>GMRPALYFCGSIRGGREDRTLYERIVSRLRRFGTVLTEHVAAAELGARGEEAAGGDRLIHEQNLEWLQQADVVVAEVTQPSLGVGYELGRAVAFNKRILCLFRPQSGRVLSAMIRGAADGSRFQVWDYEEGEV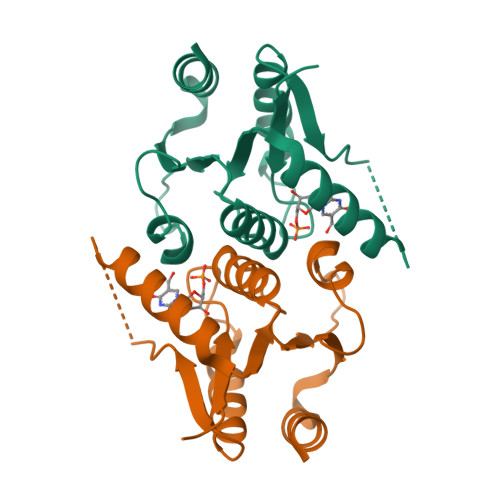EALLDRYFEADP[3x]> SRCQGKSSWPQLVGSTGAAAKAVIERENPRVRAVIIKVGSGATKDFRCDRVRVWVTE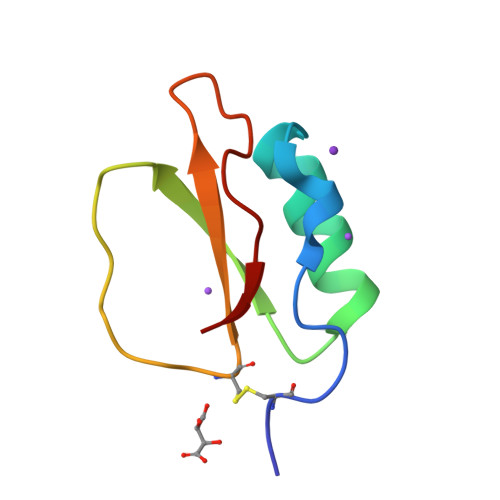RGIVARPPTIG>[2x]MAHHHHHHVGTFENITAAPADPILGLADLFRADERPGKINLGIGVYKDETGKTPVLTSVKKAEQYLLENETTKNYLGIDGIPEFGRCTQELLFGKGSALINDKRARTAQTPGGTGALRVAADFLAKNTSVKRVWVSNPSWPNHKSVFNSAGLEVREYAYYDAENHTLDFDALINSLNEAQAGDVVLFHGCCHNPTGIDPTLEQWQTLAQLSVEKGWLPLFDFAYQGFARGLEEDAEGLRAFAAMHKELIVASSYSKNFGLYNERVGACTLVAADSETVDRAFSQMKAAIRANYSNPPAHGASVVATILSNDALRAIWEQELTDMRQRIQRMRQLFVNTLQEKGANRDFSFIIKQNGMFSFSGLTKEQVLRLREEFGVYAVASGRVNVAGMTPDNMAPLCEAIVAVL

E. coli aspartate aminotransferase (AAT) is a pyridoxal phosphate (PLP)-dependent enzyme that catalyses the reversible transamination of l-aspartate with α-ketoglutarate, yielding oxaloacetate and l-glutamate. During its catalytic cycle, AAT undergoes hinge movement to switch between an open conformation, in the ligand-free form, and a closed conformation upon association with substrates or inhibitors. Using our approach, we enrich the less populated but catalytically active closed conformation in order to increase catalytic efficiency (kcat/KM) with the non-native substrate l-phenylalanine, leading to altered substrate selectivity. Steady-state kinetics reveal kcat/KM increases of up to 100-fold towards this aromatic amino acid, resulting in a selectivity switch of up to 1900-fold, and structural analyses by room-temperature X-ray crystallography and multitemperature nuclear magnetic resonance (NMR) spectroscopy confirm that the conformational landscape is remodeled to favor the target state.

To obtain structures in the absence of maleate, we applied a rigorous crystal soaking method to serially dilute and extract the inhibitor from the crystallized enzymes. Upon soaking crystals of the WT enzyme to remove the bound inhibitor, we observed that one subunit (chain A) within the enzyme homodimer was in the open conformation, confirming that the soaking procedure was able to remove the bound maleate, and that the crystal lattice could accommodate the domain rotation required for opening and closing of this subunit. Chain B however remained closed upon maleate removal, likely due to crystal packing interactions hindering domain rotation of this subunit. These results are consistent with a previous study that showed that only one subunit of a homologous AAT closed upon soaking of the crystal in a substrate solution. Overlay of AAT structures (Chain A) in the presence and absence of maleate show transition from open to closed states upon inhibitor binding for WT, VFCS, and AIFS, but not for HEX, VFIT, and VFIY, which already adopt the closed conformation in the absence of bound inhibitor. Furthermore, DynDom analyses of all variants confirmed that only WT, VFCS, and AIFS undergo hinge motion upon maleate binding, which rotates the moving domain relative to the fixed domain by 4.6, 2.6, and 5.9 degrees, respectively.D7 proteins are among the most abundant components in the salivary glands of several blood-feeding arthropods and are distantly related to the arthropod odorant-binding protein superfamily. The D7 proteins act as kratagonists, binding and trapping agonists of hemostasis, including biogenic amines and leukotrienes (LT). CxD7L1 binds adenosine 5′-monophosphate (AMP), adenosine 5′-diphosphate (ADP), adenosine 5′-triphosphate (ATP), and adenosine, which are essential agonists of platelet aggregation and act as inflammatory mediators. Taken all together, we demonstrated that CxD7L1 inhibits platelet aggregation by sequestering ADP, which is released from platelet dense granules upon platelet activation promoting a stable platelet response.

To further characterize the mechanism of the adenine nucleoside/nucleotide D7 binding, we solved the crystal structure of CxD7L1 in complex with ADP. A crystal of CxD7L1 that belonged to I212121 space group and diffracted to 1.97 Å resolution was used to collect a data set. The CxD7L1 protein fold consists of 17 helical segments stabilized by five disulfide bonds linking C18 with C51, C47 with C104, C154 with C186, C167 with C295, and C228 with C242. The structure revealed that the ligand-binding site is located between the N-terminal and C-terminal domains. The residues involved in binding ADP or stabilizing the binding pocket are S130, R133, Y137, K144, K146, N265, Y266, S263, S267, and R271. The hydrogen bonds between the adenine ring and residues Y137, K144, and Y266 determine the specificity for adenine and the lack of binding to other nucleotides with other nitrogenous bases (5′-GTP and 5′-TTP). Similarly, S267 and N265 of CxD7L1 are involved in binding to the ribose, which is possible when the phosphate group occupies position 5′ but not position 3′ or the cyclic form, as shown by calorimetry experiments. R133 binds to the oxygen of the beta phosphate of ADP which may explain the similar binding affinities for both ATP and ADP while affinity for AMP is lower as it lacks the beta phosphate. The amino acids that constitute the ADP binding pocket in CxD7L1 create a strongly negative surface, showing an inverted pattern of amino acid charges that completely change the nature of the binding pockets. Moreover, the structure of the complex CxD7L1-ADP was solved, showing a different binding mechanism for a D7 with the binding pocket located between the N-terminal and C-terminal domains whereas most D7s bind ligands within one of these two respective domains.

> DEWSPMDPEEVAFEEAKCMEDHFGNDFGLAEKWMKWSLAESDGKTACYVKCLVEALGMYDKQAFQPNNIKQQYEAYKSDNGVDQTKGDAIANELGKIDAKDGKCESIAKGFIQVNNANKGVLEKIYLLDSSVRDAIYKKNPQIKPKGISIFRFCGKQFYQDGEAAYCNVRKHGFSDDPKFIKHSNCTTRGMRWMKKNGEMDESAILRGLHAVNENGKDDVVKKSLQNCKAKDESKARDYYKCIYDGLGEQLFMKVLDYIEVRSENYSYRLREATSKYDANAMRSKVKALDSEAKC>GAMGSMSVSEANGTETIKPPMNGNPYGPNPSDFLSRVNNFSIIESTLREGEQFANAFFDTEKKIQIAKALDNFGVDYIELTSPVASEQSRQDCEAICKLGLKCKILTHIRCHMDDARVAVETGVDGVDVVIGTSQYLRKYSHGKDMTYIIDSATEVINFVKSKGIEVRFSSEDSFRSDLVDLLSLYKAVDKIGVNRVGIADTVGCATPRQVYDLIRTLRGVVSCDIECHFHNDTGMAIANAYCALEAGATHIDTSILGIGERNGITPLGALLARMYVTDREYITHKYKLNQLRELENLVADAVEVQIPFNNYITGMCAFTHKAGIHAKAILANPSTYEILKPEDFGMSRYVHVGSRLTGWNAIKSRAEQLNLHLTDAQAKELTVRIKKLADVRTLAMDDVDRVLREYHADLSDADRITKEASA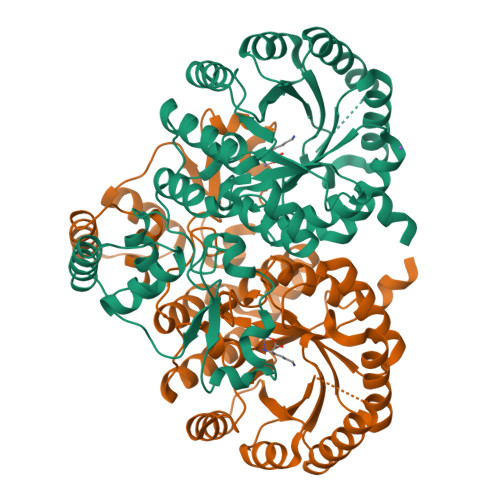[2x]> GPHMGTSARDLLREMARDKPRLLAALEVASAAMAKEEAAGGEQDALDLYQHSLGELLLLLAAEPPGRRRELLHTEVQNL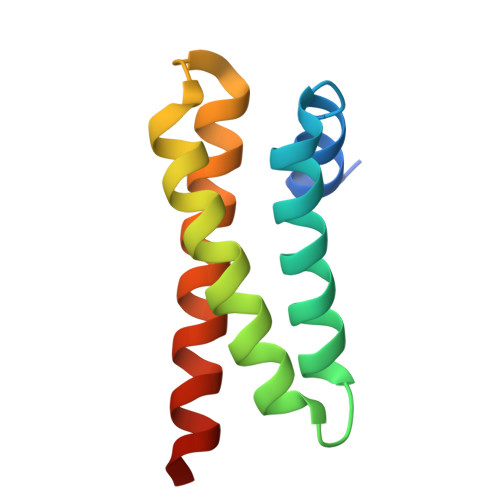MARAEYLKEQVKMRES>[3x]MKIEEVKSTTKTQRIASHSHVKGLGLDESGLAKQAASGLVGQENAREACGVIVELIKSKKMAGRAVLLAGPPGTGKTALALAIAQELGSKVPFCPMVGSEVYSTEIKKTEVLMENFRRAIGLRIKETKEVYEGEVTELTPCETENPMGGYGKTISHVIIGLKTAKGTKQLKLDPSIFESLQKERVEAGDVIYIEANSGAVKRQGRCDTYATEFDLEAEEYVPLPKGDVHKKKEIIQDVTLHDLDVANARPQGGQDILSMMGQLMKPKKTEITDKLRGEINKVVNKYIDQGIAELVPGVLFVDEVHMLDIECFTYLHRALESSIAPIVIFASNRGNCVIRGTEDITSPHGIPLDLLDRVMIIRTMLYTPQEMKQIIKIRAQTEGINISEEALNHLGEIGTKTTLRYSVQLLTPANLLAKINGKDSIEKEHVEEISELFYDAKSSAKILADQQDKYMK;>[3x]MATVTAT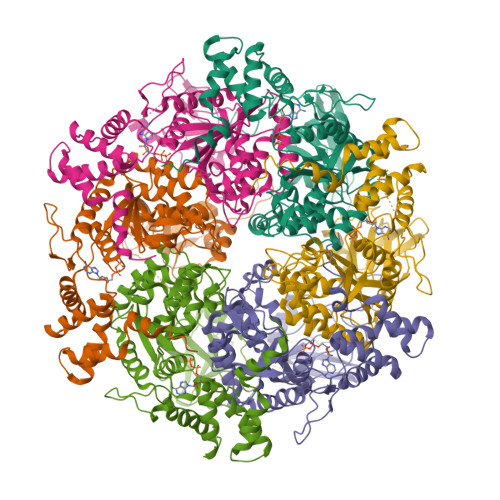TKVPEIRDVTRIERIGAHSHIRGLGLDDALEPRQASQGMVGQLAARRAAGVVLEMIREGKIAGRAVLIAGQPGTGKTAIAMGMAQALGPDTPFTAIAGSEIFSLEMSKTEALTQAFRRSIGVRIKEETEIIEGEVVEIQIDRPATGTGSKVGKLTLKTTEMETIYDLGTKMIESLTKDKVQAGDVITIDKATGKISKLGRSFTRARDYDAMGSQTKFVQCPDGELQKRKEVVHTVSLHEIDVINSRTQGFLALFSGDTGEIKSEVREQINAKVAEWREEGKAEIIPGVLFIDEVHMLDIESFSFLNRALESDMAPVLIMATNRGITRIRGTSYQSPHGIPIDLLDRLLIVSTTPYSEKDTKQILRIRCEEEDVEMSEDAYTVLTRIGLETSLRYAIQLITAASLVCRKRKGTEVQVDDIKRVYSLFLDESRSTQYMKEYQDAFLFNELKGETMDTS> HHHHHMTKNYTEAQLKYYDANTGLCGIGIDQWFQYEPERNQFSTAFPLLFMLSELSLNSKEDTTAELYKNLNLRSEDEVVNVNQAVNTNLNTKNEVYQSTLILNAYTDIDSPFSETFIQNFAKVFNGTVKNIDYSNDAVATIRDSLQSDSGNDIEIALKDGDINKDTGIILTAYTNIYFPW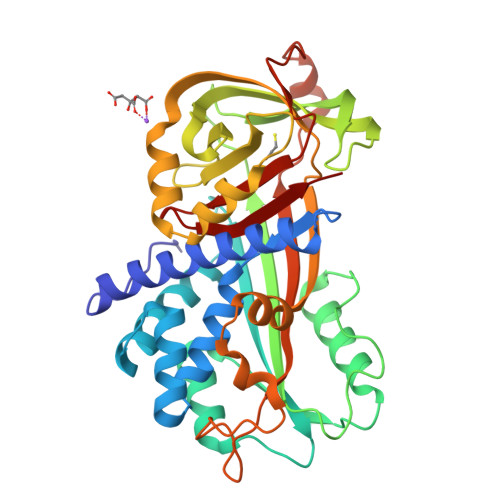GEASDSYRPYKQIDISFTALDGTQSNKQAWYSEGAGKYAEIENLGIKVFQFSLKPGLTVVLGTSLNDNNDLSGAFNKLRDPATLAYILTQTESKYLKLAVPIELTMRDSRDYIPEVKRAGLLTELFEKNFDGFDTVYDNKSGYISYMLSHTRLEFEQPTEEQAASVVAEPDFIFDKPYFFLVLDQFNTPAFIGLITN> AMGDVSYIVDSLGLPPFSYQMSLLSFTEKGPQELLQLLSDVFSTISPKHQKVDVAKEVPDQTADRLIGFLKIIKYRPNVQDPLLFRQLVAAGDRETLYQ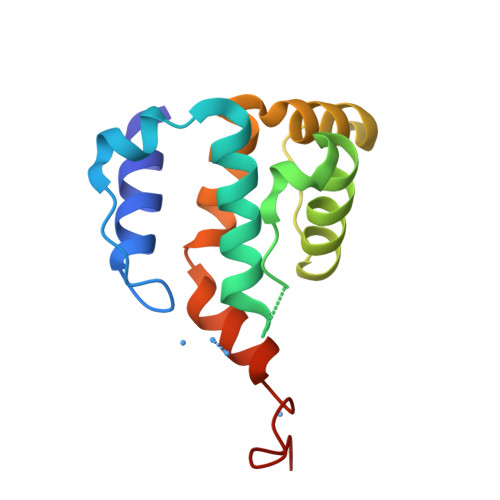ILRWVVPQAQLLEKRAFVGYYLSFPDMP> GPYASLTEIEHLVQSVCKSYRETC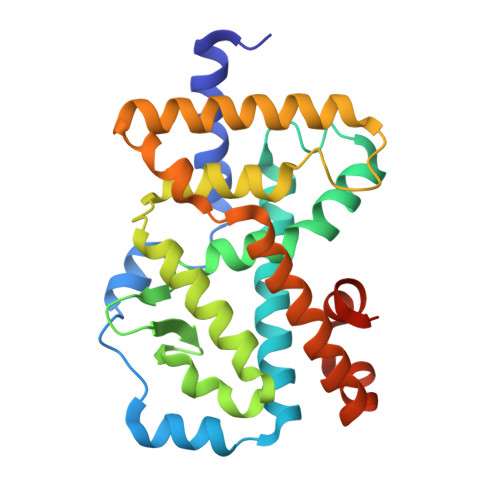QLRLEDLLRQRSNIFSREEVTGYQRKSMWEMWERCAHHLTEAIQYVVEFAKRLSGFMELCQNDQIVLLKAGAMEVVLVRMCRAYNADNRTVFFEGKYGGMELFRALGCSELISSIFDFSHSLSALHFSEDEIALYTALVLINAHRPGLQEKRKVEQLQYNLELAFHHHLSKTHRQSILAKLPPKGKLRSLCSQHVERLQIFQHLHPIVVQAAFPPLYKELFSTETESPVGLSK methyl 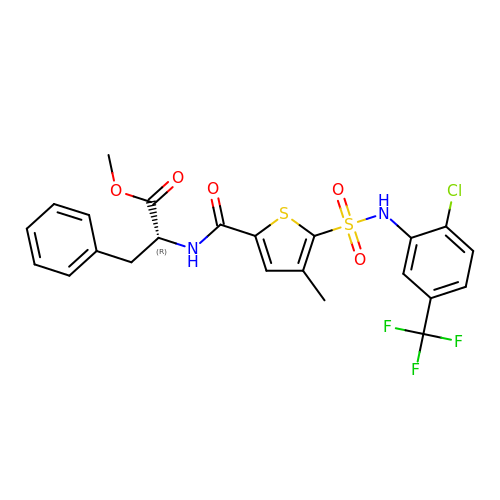N-(5-{[2-chloro-5-(trifluoromethyl)phenyl]sulfamoyl}-4-methylthiophene-2-carbonyl)-D-phenylalaninate | C23 H20 Cl F3 N2 O5 S2 | YYXGZAWTALWJLJ-GOSISDBHSA-N>[2x]MPFTYSIEATRNLATTERCIQDIRNAPVRNRSTQFQLAQQNMLAYTFGEVIPGFASAGINGMDYRDVIGRPVENAVTEGTHFFRDDFRVDSNAKAKVAGDIFEIVSSAVMWNCAARWNSLMVGEGWRSQPRYSRPTLSPSPRRQVAVLNLPRSFDWVSLLVPESQEVIEEFRAGLRKDGLGLPTSTPDLAVVVLPEEFQNDEMWR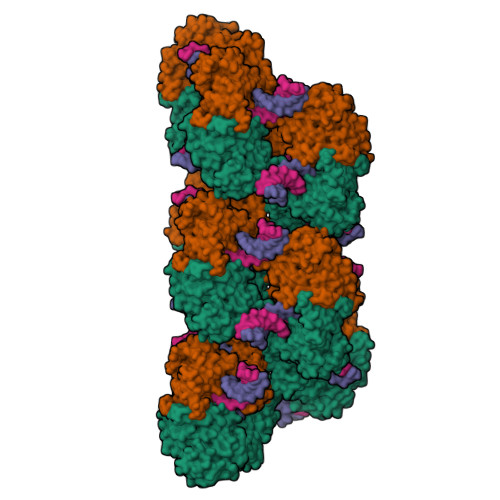EEIAGLTRPNQILLSGAYQRLQGRVQPGEISLAVAFKRSLRSDRLYQPLYEANVMQLLLEGKLGAPKVEFEVHTLAPEGTNAFVTYEAASLYGLAEGRSAVHRAIRELYVPPTAADLARRFFAFLNERMELVNG>[2x]MGHHHHHHHHHHMSKQQIGVVGMAVMGRNLALNIESRGYTVSIFNRSREKTEEVIAENPGKKLVPYYTVKEFVESLETPRRILLMVKAGAGTDAAIDSLKPYLDKGDIIIDGGNTFFQDTIRRNR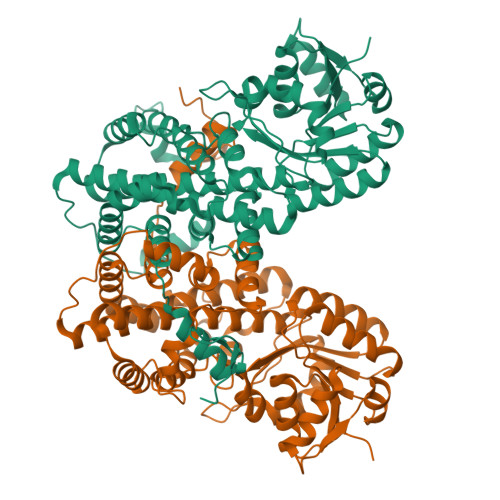ELSAEGFNFIGTGVSGGEEGALKGPSIMPGGQKEAYELVAPILTKIAAVAEDGEPCVTYIGADGAGHYVKMVHNGIEYGDMQLIAEAYSLLKGGLNLTNEELAQTFTEWNNGELSSYLIDITKDIFTKKDEDGNYLVDVILDEAANKGTGKWTSQSALDLGEPLSLITESVFARYISSLKDQRVAASKVLSGPQAQPAGDKAEFIEKVRRALYLGKIVSYAQGFSQLRAASEEYNWDLNYGEIAKIFRAGCIIRAQFLQKITDACAENPQIANLLLAPYFKQIADDYQQALRDVVAYAVQNGIPVPTFSAAVAYYDSYRAAVLPANLIQAQRDYFGAHTYKRIDKEGVFHTEWLD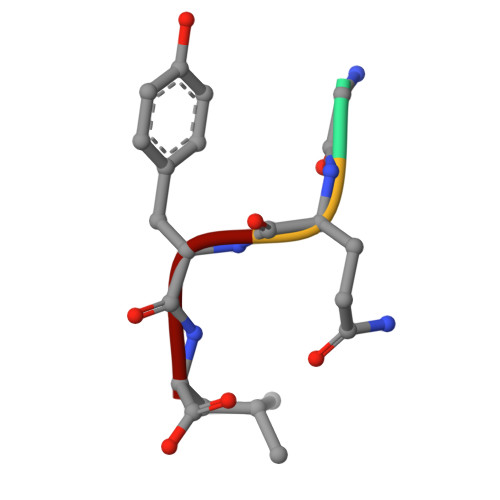> GQYL>ALPPVAKAAQVVNQTLQLDDSYPDLDSYCRPGASSDYEMQSSDSSWAPFHVVRHHNIPDKVFEHLNAGEVFTKLGLFAEIGYAWASIDSSLFLWDYTHPNPELIGYEEATHTITAVALVPPKPGVFVKTITHVLVVATTSEIILLGVSATPTPSGSKSLTLYSTRMSVHRGGSDVSFIVGTKDGRIFLGGESDTDIHEIFYQQEERWFSSRCGKINHSHPFGSRQQEWLRGLYVDDTRNLLYSLSNRSTIRTYHMEGPEKLTKVIEKDKTSCLRDFAHMADSSPLFTDKTNIVALSPIPATEASKLHLMALTDTGCRLFLSATSSASYTMGGATALAPQSMQLQFVKFPPRESPTRIRTLNGQIIDSQLDKTSRALDPSALGFRFSPGYFFDVVRKHPNQDMLFVSAPDTGRIKVTQPASALKYFEQGTWIELENGNRTIEIGLTTAPFAAAKQPLGFGNELAVQFDQVPGEFAVLTNTGVHIVRRRRLVDIFAKALGNCVSASDDALEREVRKFINQYGRVETIAAALAVACGQGSDLRTGTGRGMDRNTENLARAAFIEYGGQPRLAESDGKQSVSESVRLSSRHDALALYLTRLVRTLWKAKVVQVGSGSDISSTIPTSKLVTIQENVERLRNFLEANKSTIQGLAPPSERLFGRQEDIANQKEHQALHALQKLMESISEGISFVLMLFDERVSDIYARLDAVSQQQLKDLTYEQLFSQTPGKELAKVLVKAIVNRNIASGANVETVADALRRRCGSFCSPDDVVTFKAQEQLQRASEQAHNSPVLRALLAESLRLFEQVAGSLTPANLTTAVEQYISLKYYAGAIQLCLTVAQQKDRGNTALSWVNDGKPANDSRKKAFDERKICYNLIHQVLDKLESDFAGEPELVDGRPTLAATKRMEAYNVVNDSSDEVFHFDLYEWYIEKGWTDRILSIDSPHVITYLQRLAETDFRHAELLCRFYTTRSRFFEAAQVQTNLAKSDLNISLKDRIILLSRAKGNASVNTIGISRQQQQQLNHEASELLEIAHIQDDLLERLVADPRIPEERKAEIEEFLDGPIRTLTDLFNDYADQANYYDLCLLIFHAADFHNPRTILDTWNNLINQSHFEAEQRREYWEIVQAGGDLPAGVIAPIAEPPLPYVYVSQQIQLIAHRTSLDSLIFPVNSLLPVVCAYAINNGQDASIGADPCWPIQLFLNLGVPHALVVQVLENVLDTQEAPFTGRRRKLVVQWIAMAVDMWVREVERRGAMAAAAASGASGSEAVMGSWVSELLGRADQVLTQIAGTGATLRGGAASDAEEIASLRRTVKGLKRSVD[2x];>DLPPVAKAAQVVNQTLQLDDSYPDLDSYCRPGASSDYEMQSSDSSWAPFHVVRHHNIPDKVFEHLNAGEVFTKLGLFAEIGYAWASIDSSLFLWDYTHPNPELIGYEEATHTITAVALVPPKPGVFVKTITHVLVVATTSEIILLGVSATPTPSGSKSLTLYSTRMSVHRGGSDVSFIVGTKDGRIFLGGESDTDIHEIFYQQEERWFSSRCGKINHSHPFGSRQQEWLRGLYVDDTRNLLYSLSNRSTIRTYHMEGPEKLTKVIEKDKTSCLRDFAHMADSSPLFTDKTNIVALSPIPATEASKLHLMALTDTGCRLFLSATSSASYTMGGATSLAPQSMQLQFVKFPPRESPTRIRTLNGQIIDSQLDKTSRALDPSALGFRFSPGYFFDVVRKHPNQDMLFVSAPDTGRIKVTQPASALKYFEQGTWIELENGNRTIEIGLTTAPFAAAKQPLGFGNELAVQFDQVPGEFAVLTNTGVHIVRRRRLVDIFAKALGNCVSASDDALEREVRKFINQYGRVETIAAALAVACGQGSDLRTGTGRGMDRNTENLARAAFIEYGGQPRLAASDGKQSVSESVRLSSRHDALALYLTRLVRTLWKAKVVQVGSGSDISSTIPTLVTIQENVERLRNFLEANKSTIQGLAPPSERLFGRQEDIANQKEHQALHALQKLMESISEGISFVLMLFDERVSDIYARLDAVSQQQLKDLTYEQLFSQTPGKELAKVLVKAIVNRNIASGANVETVADALRRRCGSFCAPDDVVTFKAQEQLQRASEQAHNAPVLRALLAESLRLFEQVAGSLTPANLTTAVEQMISLKYYAGAIQLCLTVAQQKDRGNTALSWVNDGKPANDSRKKAFDERKICYNLIHQVLDKLESDFAGEPELVDGRPTLAATKRMEAYNVVNDSSDEVFHFDMYEWYIEKGWTDRILSIDSPHVITYLQRLAETDFRHAELLCRFYTTRSRFFEAAQVQTNLAKSDLNISLKDRIILLSRAKGNASVNTIGISRQQQQQLNHEASELLEIAHIQDDLLERLVADPRIPEERKAEIEEFLDGPIRTLTDLFNDYADQANYYDLCLLIFHAADFHNPRTIMDTWNNLINQSHFEAEQRREYWEIVQAGGDLPAGVIAPIAEPPLPYVYVSQQIQLIAHRTSLDSLIFPVNSLLPVVCAYAINNGQDASIGADPCWPIQLFLNLGVPHALMVQVLENVLDTQEAPFTGRRRKLVVQWIAMAVDMWVREVERRGAMAAAAASGASGSEAVMGSWVSELLGRADQVLTQIAGTGATLRGGAASDAEEIASLRRTVKGLKRSVDMLLGGEMARMSFFR[2x];>[2x]DLPPVAKAAQVVNQTLQLDDSYPDLDSYCRPGASSDYEMQSSDSSWAPFHVVRHHNIPDKVFEHLNAGEVFTKLGLFAEIGYAWASIDSSLFLWDYTHPNPELIGYEEATHTITAVALVPPKPGVFVKTITHVLVVATTSEIILLGVSATPTPSGSKSLTLYSTRMSVHRGGSDVSFIVGTKDGRIFLGGESDTDIHEIFYQQEERWFSSRCGKINHSHPFGSRQQEWLRGLYVDDTRNLLYSLSNRSTIRTYHMEGPEKLTKVIEKDKTSCLRDFAHMADSSPLFTDKTNIVALSPIPATEASKLHLMALTDTGCRLFLSATSSASYTMGGATALAPQSMQLQFVKFPPRESPTRIRTLNGQIIDSQLDKTSRALDPSALGFRFSPGYFFDVVRKHPNQDMLFVSAPDTGRIKVTQPASALKYFEQGTWIELENGNRTIEIGLTTAPFAAAKQPLGFGNELAVQFDQVPGEFAVLTNTGVHIVRRRRLVDIFAKALGNCVSASDDALEREVRKFINQYGRVETIAAALAVACGQGSDLRTGTGRGMDRNTENLARAAFIEYGGQPRLAESDGKQSVSESVRLSSRHDALALYLTRLVRTLWKAKVVQVGSGSDISSTIPTSKLVTIQENVERLRNFLEANKSTIQGLAPPSERLFGRQEDIANQKEHQALHALQKLMESISEGISFVLMLFDERVSDIYARLDAVSQQQLKDLTYEQLFSQTPGKELAKVLVKAIVNRNIASGANVETVADALRRRCGSFCSPDDVVTFKAQEQLQRASEQAHNSPVLRALLAESLRLFEQVAGSLTPANLTTAVEQMISLKYYAGAIQLCLTVAQQKDRGNTALSWVNDGKPANDSRKKAFDERKICYNLIHQVLDKLESDFAGEPELVDGRPTLAATKRMEAYNVVNDSSDEVFHFDMYEWYIEKGWTDRILSIDSPHVITYLQRLAETDFRHAELLCRFYTTRSRFFEAAQVQTNLAKSDLNISLKDRIILLSRAKGNASVNTIGISRQQQQQLNHEASELLEIAHIQDDLLERLVADPRIPEERKAEIEEFLDGPIRTLTDLFNDYADQANYYDLCLLIFHAADFHNPRTIMDTWNNLINQSHFEAEQRREYWEIVQAGGDLPAGVIAPIAEPPLPYVYVSQQIQLIAHRTSLDSLIFPVNSLLPVVCAYAINNGQDASIGADPCWPIQLFLNLGVPHALMVQVLENVLDTQEAPFTGRRRKLVVQWIAMAVDMWVREVERRGAMAAAAASGASGSEAVMGSWVSELLGRADQVLTQIAGTGATLRGGAASDAEEIASLRRTVKGLKRSVDMLLGGEMARMSFFR;>[6x]RKAKLLPMEEALLP;>[6x]HKKLVINKDMRTDLFSPPN;>[7x]SSLDNIEMAYARQIYIYNEKIVNGHLQPNLVDLCASVAELDDKSISDMWTMVKQMTDVLLTPATDALKNRSSVEVRMEFVRQALAYLEQSYKNYTLVTVFGNLHQAQLGGVPGTYQLVRSFLNIKLPAPLPGLQDGEVEGHPVWALIYYCMRCGDLLAASQVVNRAQHQLGEFKTWFQEYMNSKDRRLSPATENKLRLHYRRALRNNTDPYKRAVYCIIGRCDVTDNQSEVADKTEDYLWLKLNQVCFDDDGTSSPQDRLTLSQFQKQLLEDYGESHFTVNQQPFLYFQVLFLTAQFEAAVAFLFRMERLRCHAVHVALVLFELKLLLKSSGQSAQLLSHEPGDPPCLRRLNFVRLLMLYTRKFESTDPREALQYFYFLRDEKDSQGENMFLRCVSELVIESREFDMILGKLENDGSRKPGVIDKFTSDTKPIINKVASVAENKGLFEEAAKLYDLAKNADKVLELMNKLLSPVVPQISAPQSNKERLKNMALSIAERYRAQGISANKFVDSTFYLLLDLITFFDEYHSGHIDRAFDIIERLKLVPLNQESVEERVAAFRNFSDEIRHNLSEVLLATMNILFTQFKRLKGTSPSSSSRPQRVIEDRDSQLRSQARTLITFAGMIPYRTSGDTNARLVQMEVLMN;>APPVRSIY[7x];>[2x]MATLTDRTYLPPLEDCLTGRTVILSWRLVASALEDADLARLTSPALSTFLRDGFVHELLKHPARVFEPKDLKQEFETKTSSIQTVAPGVDTIKKDALWLADAVAINQVAALRIVLIEYQTRAHSHLVLPLSTQDVANIQEAAGVGDAHASSILSLLNPASAVDAETMWCDFETEARRRERILATYLSERRSFTAAVDALVTFLLHSAPGQHKDLDSLRRALLKDAFAFDEDLDVPDRSKLLTMAPTYMNLVEDCIARAQALPAKLGESFKTEAFELDWLRTAITEAVHSLSIAFQALDLDTPYFAPHELLSEWFELMNSSLFLESILGFEVVADLAMPARSLVSAICLKMLNIDRTIQFLHDFDYPDGEEPYLLSSQTLNKIHTAVTNAVNSGVAASLPVAFAWSLIVHQMHLGYQERAERRDLLVNQRAQAGFELEFQPSASTPNRRRRNSAGSIVSLEASPYDDFLREQRLDNDIAPVEQIAMLATSRGQVYQVMSEMALCLGTTHEAAFRPAVGARARLVFQDLLKRAAYLIPYQDEPVFSLLAILATGRQYWDVTDALSASSLNQVYTDMLDDETLFTQFTMQAINRFPYEFNPFSVLCRVLAAALITNKDKADVVTGWLWRTPTLTVDWNPAWDRSYELCFEDENTNSFRLTRDVDLFGSASPARPRHLAAEERFIIPEGTLGRFVTDVGRTARLEFEHSALALLGKRLEVKAAEEICDSGMAPLDVDEQAEAVAMLATVLRAESLKSTAKGGDPEAPLKFLKEASRLLPHNKDILTVISDTIDGLVEKELLELDGPQIAVLASCLQFLHAALAVCPGRVWAYMSRCALIAGDARPGRLSRITGSLDMYAERFDLLSSAVKLFAALIDSAACSAVQRRAGSTALVSVRSAVENPWLGTSEKILSRVALAIAQAALDVYESTTTWRFRSELDRSILVRDVVGLMHKLVVHAHTLSSHLTSTLSPAAAHIISSFLTPPPSASSLRFQPLLGTLLVALITPRATLYPGQSRILAERVTSVLAFCTSLLRAADFLGQTHIPLQTHLFQSACLLARLPAANAVYRAPVLELLRALVEVAGRAANGSGEPPSLLGYLGSHAARSFISLVEGIDKPFGRVEHAVVTWRFFAAVIRNRQQWMAGCLLTGRTPREALKGGGEQKIERKVGEGSVLAAAMERLREVKSLDVQEAVAVMDFVVSAQNYWPWTIFAVRKEKEVVDALRGYVRGLKAPGMVMKTDGAAAAAFQARIAAYVAETFAMQLYHMRQMRQAEKFAGELVADLDYFLREGVMVWGYNASLHGNFARNFAKRFPGVEVDDFKRTMWLPRELGKGYYYALEVAEQMLGFDAGWGGVKQSGFRKEMETANLNLSLVEAQVSLFHAWEYLLLELTLSLLPKKENAAFARQVLQVVEQCLEANQRSQPPENIFVVLGHARAGLALTLLQRLADANQLPRDVTHLLALVSSAIHAVENPFGANDLPYFRTLLKILFVVLRAAKQGTAKPGESNVAITQQVLTILDRVVARCFRALAALVHEQQQNATDGTTTAPEDLALITAILQACLSVPGIEQCQVQVLNIMAAHDVFQVAVALFSWADRLLPANPSPASSSTSTSATNPASGDPVYGELALLFLLELSALPALAEHLACDGLLGHLAAARLAGYMRRTNVGPFAENAGAARCYAIWAKCLLPLLLNILAALGSTVAPEVAWVLNQFPNLLQSSVERIEPPGFSRPTLSLASTPPRQKFISLLEISEIHSLALLTRVLAACRAQNARDVPEVTWDGAKVLECVEYWLRGRKVLRERLVPLGPREVEWRGMVATGGVVGVAGDGGEGCENRLEEKAVGLLVGVREVLEGGLEGEGE;>[2x]DVDTYLSNLQTKTTLSMIADGLERSARDFDAFLEENVTLEWEAQRKRIYQHFG;>[2x]EDSILQPGAFSAN;>MTDLRKLEALQALHAELVAVRQHRFEGLQVLETLLEEQTDAFKALIAKPARDTKDREALGKEPKKLKIGEEEYSLNEDFVNDCLKLADELDLNEKESARILIDCDAEGDVETQSRPLWECGVIRFHQERKYLLDCMRLILEIAADEDIDAGLQESFGVAAEDKIFGIPPPWERNKENQPTQVKKFIPRCMEAMKGVRSMLQCMADKANARNMLQQASLVRPLDNQETLDFSRLSLVEQHECLASILHAAVQRHHATIADFQDFIKILRKWDKYDHFLIHLIPVLAAYITEFGSPEGMGDLQQARRLNDFICKGGDEDSWALPVLGAAVRAWWIAEHNGFYLDDTVQDLRGINLDEEDEQRTKQFLDALKEGAFDFILSVAADCKAQEWQDPSQLGARQWLQRKIPSLPSEPFPFSHFLQHSLMVHLEGFVDATISNLPDVLRKLRTEEDEQRQLRPNHEQDMDLERFLIIISYAYEGRPDAAMSFWEDPDSNLAGFLQWASRRASTPLVSAFCEMLRCLADNEECATAAHNFLLDEGHQASGKMKRSQSLTWSQIFKELEYFTTKVCSERPNPPQASMHRPGRPGADPAEIEPESALMLECYLRLIAKLATESEIARKRLIMDEDFNLVDTILKLSVGVIPHRLRACIFYVLKALMIRKTHEELDAMWRWVEAWMTNPFSSLPGSQGAPQRISFLGQTPGPQECMEMMFREFGTGFEQSNAFIQLLTTLLVPPEGLNSLNDSVPFPEWLGSSIRTLGIEPYVDFVFDVFANRTKDISDPSQLRILRLSCLDFVMVCLVTFNEDLIVLGHESNISIDDAMAATNLATYVRLHPFSRVMEWLFNEKVITSLINTIHQDPISLGSASPDSPLVVSILRAIQVMIKALELQETYLHLVRPEVLRYQGEAGVRRKPVANAAYSAFEDGILSHLSLVVDLGKYCNLGHAELTLACLKLLEKISTSSRILSAWSPDSGRLGHRNKAIVQLERNGEGETISASLSASIMATLDPALAASGENYRVKLAILDFLYACLRATPDQPTIAHQLLGFHCELSKLGIEPKGPFDMQKSLFHSLLNVLITLTVSEEEQGMRGYLVTLKYRVLRILQLLWKSPLSASLVMDELRATNFLFHMLLREVQIQPQLPWDGQLVTGCEFLLSDASLAYIDYLASRAAIFEYIGKELCSVSQNRIPSIKRQIFDALNGQIFVDEEAPLTIPSIFDFFDFINTDYKWEEIPSPHFTYLKDLDLGPCILEHKYAGVHYDIRKAQEILALKRKEYEHSQLATPEFLETVELEEKVLIEWLTVRNRANLLLTARLNLLQAWANLLLVMIESNDFKSTPKMAFLLQALQAILPTLEAFSSLKSDEAFELARVAKVLLWKLDFSQDSDAGLDREQFTVGNLIGDKLFQLFQLCLSAISQCSGTPELRSLYYSICYRYLTAVVDNDATVAATPASSTIGPTRSVTNARARTLKAITLYGDRLLNVICDDAYGSDTTCQTAAMILLNALVHTSRASSAAGVSPADVDCPIIDALNRLNFIGVLVDSLKEILNEWLAPSSTFDPSLSTNASPSLPIPASPSQQYTSAKLALLLQLCQTRQGAKYVLQANLFRALEQSGVFAADPELVEVDSESGVPRVVALERHYALLVALARVVGAAVTARGAHNIVQGRKFLTQHRGLVVHVLKKNAGIGGGVVGNSLASSINGGSTATMTRRDEILAQQALEERIEELAEAFMLLITATGFLEYESEQVPSEQPRAHTTFFH[5x];>[5x]SGTGLGEVDVDTYLSNLQTKTTLSMIADGLERSARDFDAFLEENVTLEWEAQRKRIYQHFGIK;>ILPMYKLSP[5x];>FG[5x];>MDEIITRWATDLAKYQKEFKEQAAKVMEWDRLLVENGEKIQKLYTSTYEAERASNEIERQLSNVESQQEELTAWLDRYERELDELYAKQMGSAAGEQAAGPDQERERTYKLAEKLTDQLDEMGKDLAKMIKEINDMSNTLSKGSKPDDPLTQIVRVLNGHLAQLQWIDTNAAALQAKVAAAQK[4x];>SEALQQEIAKIDEEIQKCIRDKEAVDAFLPAHGEQLAAIPTDVNFVTRKSEGAHNALSSDILAIDQLRELVKQDADNARLSFKAIDNLKLPMQYHQAGLWSKQMGGAGTAGASGASADADGQSNADLISYFSKTADEMEEMMKKFEKTITEIEAHLTGVEAHAMAMQNVAAQSRNAAQGGVDERVYELAAVLREFEESILKVAGVVGGVKEGVTELQLRDFM[4x];>[4x]PIPEQIKLIVDKWNPNHPNCAFKTYLYNKVDEHTVPLYGPGPNEDPKEWEEALQRKPAPNFIPVLCSGFPSIVARLMLQRRVITEFNNKLHQINASLDAILSRHDLDHTVRAFNARRRHAELSRRCLHLAARVQVLRNRGYALSGDEDELKQKLQQIDKTLNDPAQGSRLEELWSRLIVLRGYAEDLKDQINQAGITESDGLGEEIEAKAKKILEDYDKQLQHLKKQVEEAKKDFEEWEKQ;>DEDGLISLIFNKKESDIRGQQQQLVESLHKVLGGHQTLTVNVEGVKTKADNQTEVIIYVVERSPNGTSRRVGASALFSYFEQAHIKANMQSLGVTGAMAQTELSPVQIKQLIQNPL[4x];>DHLDDSWVTVFGFPQASASYILLQFAQYGNILKHVMSNTGNWMHIRYQSKLQARKALSKDGRIFGESIMIGVKPCIDKSVMESS[4x];>ALFDSLLARNKKQAEGETALGELPSLQLGLADLRQRLRKL[4x];>MFPAAPSPRTPGTGSRRGPLAGLGPGSTPRTASRKGLPLGSAVSSPVLFSPVGRRSSLSSRGTPTRMFPHHSITESVNYDVKTFGSSLPVKVMEALTLAEVDDQLTINIDEGGWACLVCKEKLIIWKIALSPITKLSVCKELQLPPSDFHWSADLVALSYSSPSGEAHSTQAVAVMVATREGSIRYWPSLAGEDTYTEAFVDSGGDKTYSFLTAVQGGSFILSSSGSQLIRLIPESSGKIHQHILPQGQGMLSGIGRKVSSLFGILSPSSDLTLSSVLWDRERSSFYSLTSSNISKWELDDSSEKHAYSWDINRALKENITDAIWGSESNYEAIKEGVNIRYLDLKQNCDGLVILAAAWHSADNPCLIYYSLITIEDNGCQMSDAVTVEVTQYNPPFQSEDLILCQLTVPNFSNQTAYLYNESAVYVCSTGTGKFSLPQEKIVFNAQGDSVLGAGACGGVPIIFSRNSGLVSITSRENVSILAEDLEGSLASSVAGPNSESMIFETTTKNETIAQEDKIKLLKAAFLQYCRKDLGHAQMVVDELFSSHSDLDSDSELDRAVTQISVDLMDDYPASDPRWAESVPEEAPGFSNTSLIILHQLEDKMKAHSFLMDFIHQVGLFGRLGSFPVRGTPMATRLLLCEHAEKLSAAIVLKNHHSRLSDLVNTAILIALNKREYEIPSNLTPADVFFREVSQVDTICECLLEHEEQVLRDAPMDSIEWAEVVINVNNILKDMLQAASHYRQNRNSLYRREESLEKEPEYVPWTATSGPGGIRTVIIRQHEIVLKVAYPQADSNLRNIVTEQLVALIDCFLDGYVSQLKSVDKSSNRERYDNLEMEYLQKRSDLLSPLLSLGQYLWAASLAEKYCDFDILVQMCEQTDNQSRLQRYMTQFADQNFSDFLFRWYLEKGKRGKLLSQPISQHGQLANFLQA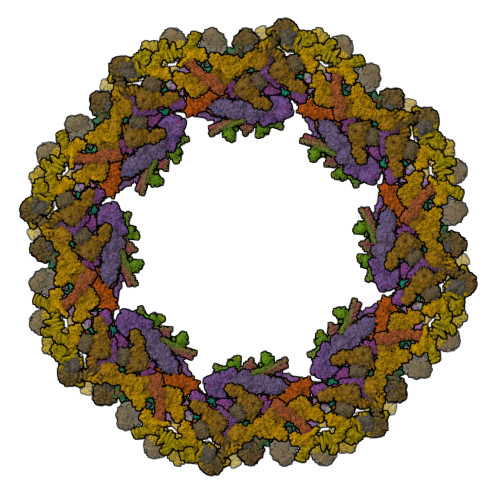HEHLSWLHEINSQELEKAHATLLGLANMETRYFAKKKTLLGLSKLAALASDFSEDMLQEKIEEMAEQERFLLHQETLPEQLLAEKQLNLSAMPVLTAPQLIGLYICEENRRANEYDFKKALDLLEYIDEEEDININDLKLEILCKALQRDNWSSSDGKDDPIEVSKDSIFVKILQKLLKDGIQLSEYLPEVKDLLQADQLGSLKSNPYFEFVLKANYEYYVQGQI[4x];>EDRLKIDVIDWLVFDPAQRAEALKQGNAIMRKFLASKKHEAAKEVFVKIPQDSIAEIYNQCEEQGMESPLPAEDDNAIREHLCIRAYLEAHETFNEWFKHMNSVPQKPALIPQPTFTEKVAHEHKEKKYEMDFGIWKGHLDALTADVKEKMYNVLLFVDGGWMVDVREDAKEDHERTHQMVLLRKLCLPMLCFLLHTILHSTGQYQECLQLADMVSSERHKLYLVFSKEELRKLLQKLRESSLMLLDQGLDPLGYEIQ[4x];>[4x]YQTERFTKFSDTLKEFKIEQNNEQNPIDPFNIIREFRSAAGQLALDLANSGDESNVISSKDWELEARFWHLVELLLVFRNADLDLDEMELHPYNSRGLFEKKLMQDNKQLYQIWIVMVWLKENTYVMERPKNVPTSKWLNSITSGGLKSCDLDFPLRENTNVLDVKDKEEDHIFFKYIYELILAGAIDEALEEAKLSDNISICMILCGIQEYLNPVIDTQIANEFNTQQGIKKHSLWRRTVYSLSQQAGLDPYERAIYSYLSGAIPNQEVLQYSDWESDLHIHLNQILQTEIENYLLENNQVGTDELILPLPSHALTVQEVLNRVASRHPSESEHPIRVLMASVILDSLPSVIHSSVEMLLDVVKGTEASNDIIDKPYLLRIVTHLAICLDIINPGSVEEVDKSKLITTYISLLKLQGLYENIPIYATFLNESDCL;>[4x]DWVEQLILAGSSLRSVFATSKEFDGPCQNEIDLLFSECNDEIDNAKLIMKERRFTASYTFAKFSTGSMLLTKDIVGKSGVSIKRLPTELQRKFLFDDVYLDKEIEKVTIEARKSNPYPQISESSLLFKDALDYMEKTSSDYNLWKLSSILFDPVSYPYKTDNDQVKMALLKKERHCRLTSWIVSQIGPEIEEKIRNSSNEIEQIFLYLLLNDVVRASKLAIESKNGHLSVLISYLGSNDPRIRDLAELQLQKWSTGGCSIDKNISKIYKLLSGSPFEGLFSLKELESEFSWLCLLNLTLCYGQIDEYSLESLVQSHLDKFSLPYDDPIGVIFQLYAANENTEKLYKEVRQRTNALDVQFCWYLIQTLRFNGTRVFSKETSDEATFAFAAQLEFAQLHGHSLFVSCFLNDDKAAEDTIKRLVMREITLLRASTNDHILNRLKIPSQLIFNAQALKDRYEGNYLSEVQNLLLGSSYDLAEMAIVTSLGPRLLLSNNPVQNNELKTLREILNEFPDSERDKWSVSINVFEVYLKLVLDNVETQETIDSLISGMKIFYDQYKHCREVAACCNVMSQEIVSKILEKNNPSIGDSKAKLLELPLGQPEKAYLRGEFAQDLMKCTYKI;>[4x]HNELIHDAVLDYYGKRLATCSSDKTIKIFEVEGETHKLIDTLTGHEGPVWRVDWAHPKFGTILASCSYDGKVLIWKEENGRWSQIAVHAVHSASVNSVQWAPHEYGPLLLVASSDGKVSVVEFKENGTTSPIIIDAHAIGVNSASWAPATIEEDGEHNGTKESRKFVTGGADNLVKIWKYNSDAQTYVLESTLEGHSDWVRDVAWSPTVLLRSYLASVSQDRTCIIWTQDNEQGPWKKTLLKEEKFPDVLWRASWSLSGNVLALSGGDNKVTLWKENLEGKWEPAG;>ILVPMTVNDQPIEKNGDKMPLKFKLGPLSYQNMAFITAKDKYKLYPVRIPRLDTSKEFSAYVSGLFEIYRDLGDDRVFNVPTIGVVNSNFAKEHNATVNLAMEAILNELEVFIGRVKDQDGRVNRFYELEESLTVLNCLRTMYFILDGQDVEENRSEFIESLLNWINRSDGEPDEEYIEQVFSVKDSTAGKKVFETQYFWKLLNQLVLRGLLSQAIGCIERSDLLPYLSDTCAVSFDAVSDSIELLKQYPKDSSSTFREWKNLVLKLSQAFGSSATDISGELRDYIEDFLLVIGGNQRKILQYSRTWYESFCGFLLYYIPSLELSAEYLQMSLEANVVDITNDWEQPCVDIISGKIHSILPVMESLDSCTAAFTAMICEAKGLIENIFEGEKNSDDYSNEDNEMLEDLFSYRNGMASYMLNSFAFELCSLGDKELWPVAIGLIALSATGTRSAKKMVIAELLPHYPFVTNDDIEWMLSICVEWRLPEIAKEIYTTLGNQMLSAHNIIESIANFSRAGKYELVKSYSWLLFEASCMEGQKLDDPVLNAIVSKNSPAEDDVIIPQDILDCVVTNSMRQTLAPYAVLSQFYELRDREDWGQALRLLLLLIEFPYLPKHYLVLLVAKFLYPIFLLDDKKLMDEDSVATVIEVIETKWDDADEKSSNLYETIIEADKSLPSSMATLLKNLRKKLNFKLCQAFM[4x];>[4x]MQPFDSGHDDLVHDVVYDFYGRHVATCSSDQHIKVFKLDKDTSNWELSDSWRAHDSSIVAIDWASPEYGRIIASASYDKTVKLWEEDPDQEECSGRRWNKLCTLNDSKGSLYSVKFAPAHLGLKLACLGNDGILRLYDALEPSDLRSWTLTSEMKVLSIPPANHLQSDFCLSWCPSRFSPEKLAVSALEQAIIYQRGKDGKLHVAAKLPGHKSLIRSISWAPSIGRWYQLIATGCKDGRIRIFKITEKLSPLASEESLTNSNMFDNSADVDMDAQGRSDSNTEEKAELQSNLQVELLSEHDDHNGEVWSVSWNLTGTILSSAGDDGKVRLWKATYSNEFKCMSVIT;>[4x]MACLSRIDANLLQYYEKPEPNNTVDLYVSNNSNNNGLKEGDKSISTPVPQPYGSEYSNCLLLSNSEYICYHFSSRSTLLTFYPLSDAYHGKTINIHLPNASMNQRYTLTIQEVEQQLLVNVILKDGSFLTLQLPLSFLFSSANTLNGEWFHLQNPYDFTVRVPHFLFYVSPQFSVVFLEDGGLLGLKKVDGVHYEPLLFNDNSYLKSLTRFFSRSSKSDYDSVISCKLFHERYLIVLTQNCHLKIWDLTSFTLIQDYDMVSQSDSDPSHFRKVEAVGEYLSLYNNTLVTLLPLENGLFQMGTLLVDSSGILTYTFQNNIPTNLSASAIWSIVDLVLTRPLELNVEASYLNLIVLWKSGTASKLQILNVNDESFKNYEWIESVNKSLVDLQSEHDLDIVTKTGDVERGFCNLKSRYGTQIFERAQQILSENKIIMAHNEDEEYLANLETILRDVKTAFNEASSITLYGDEIILVNCFQPYNHSLYKLNTTVENWFYNMHSETDGSELFKYLRTLNGFASTLSNDVLRSISKKFLDIITGELPDSMTTVEKFTDIFKNCLENQFEITNLKILFDELNSFDIPVVLNDLINNQMKPGIFWKKDFISAIKFDGFTSIISLESLHQLLSIHYRITLQVLLTFVLFDLDTEIFGQHISTLLDLHYKQFLLLNLYRQDKCLLAEVLLKDSSEFSFGVKFFNYGQLIAYIDSLNSNVYNASITENSFFMTFFRSYIIENTSHKNIRFFLENVECPFYLRHNEVQEFMFAMTLFSCGNFDQSYEIFQLHDYPEAINDKLPTFLEDLKSENYHGDSIWKDLLCTFTVPYRHSAFYYQLSLLFDRNNSQEFALKCISKSAEYSLKEIQIEELQDFKEKQHIHYLNLLIHFRMFEEVLDVLRLGHECLSDTVRTNFLQLLLQEDIYSRDFFSTLLRLCNAHSDNGELYLRTVDIKIVDSILSQNLRSGDWECFKKLYCFRMLNKSERAAAEVLYQYILMQADLDVIRKRKCYLMVINVLSSFDSAYDQWILNGSKVVTLTDLRDELRGL;>[4x]MEEIYAKFVSQKISKTRWRPLPPGSLQTAETFATGSWDNEENYISLWSIGDFGNLDSDGGFEGDHQLLCDIRHHGDVMDLQFFDQERIVAASSTGCVTVFLHHPNNQTLSVNQQWTTAHYHTGPGSPSYSSAPCTGVVCNNPEIVTVGEDGRINLFRADHKEAVRTIDNADSSTLHAVTFLRTPEILTVNSIGQLKIWDFRQQGNEPSQILSLTGDRVPLHCVDRHPNQQHVVATGGQDGMLSIWDVRQGTMPVSLLKAHEAEMWEVHFHPSNPEHLFTCSEDGSLWHWDASTDVPEKSSLFHQGGRSSTFLSHSISNQANVHQSVISSWLSTDPAKDRIEITSLLPSRSLSVNTLDVLGPCLVCGTDAEAIYVTRHLFS;>[4x]MTLSSNQYQLPLNVRPYTTTWCSQSPSCSNLLAIGHDTGITIYCASEEQTPGSTGLTLQELFTIQTGLPTLHLSFSSSCSYSENLHDGDGNVNSSPVYSLFLACVCQDNTVRLIITKNETIITQHVLGGKSGHHNFVNDIDIADVYSADNRLAEQVIASVGDDCTLIIWRLTDEGPILAGYPLSSPGISVQFRPSNPNQLIVGERNGNIRIFDWTLNLSAEENSQTELVKNPWLLTLNTLPLVNTCHSSGIASSLANVRWIGSDGSGILAMCKSGAWLRWNLFANNDYNEISDSTMKLGPKNLLPNVQGISLFPSLLGACPHPRYMDYFATAHSQHGLIQLINTYEKDSNSIPIQLGMPIVDFCWHQDGSHLAIATEGSVLLTRLMGFTRL>[4x]ARKIGIIGLGNVGAAVAHGLIAQGVADDYVFIDANEAKVKADQIDFQDAMANLEAHGNIVINDWAALADADVVISTLGNIKLQQDNPTGDRFAELK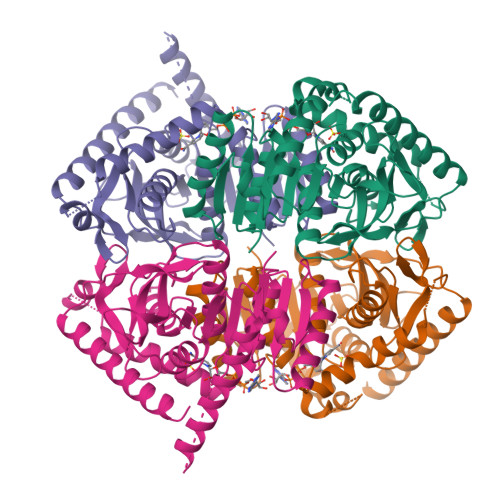FTSSMVQSVGTNLKESGFHGVLVVISNPVDVITALFQHVTGFPAHKVIGTGTLLDTARMQRAVGEAFDLDPRSVSGYNLGEHGNSQFVAWSTVRVMGQPIVTLADAGDIDLAAIEEEARKGGFTVLNGKGYTSYGVATSAIRIAKAVMADAHAELVVSNRRDDMGMYLSYPAIIGRDGVLAETTLDLTTDEQEKLLQSRDYIQQRFDEIVDTL> STDNAETGVIEAGNTDTDFSGELAAPGSNHTNVKFLFDRSRLLNVIKVLEKDAVFPRPFPTQEGAQQDDGYFCLLTPRPTVASRPATRFGLYANPSGSGVLANTSLDFNFYSLACFTYFRSDLEVTVVSLEPDLEFAVGWFPSGSEYQASSFVYDQLHVPFHFTGRTPRAFASKGGKVSFVLPWNSVSSVLPVRWGGASKLSSATRGLPAHADWGTIYAFVPRPNEKKSTAVKHVAVYIRYKNARAWCPSMLPFRSYK;> GPIPTAPRENSLMFLSTLPDDTVPAYGNVRTPPVNYLPGEITDLLQLARIPTLMAFERVPEPVPASDTYVPYVAVPTQFDDRPLISFPITLSDPVYQNTLVGAISSNFANYRGCIQITLTFCGPMMARGKFLLSYSPPNGTQPQTLSEAMQCTYSIWDIGLNSSWTFVVPYISPSDYRETRAITNSVYSADGWFSLHKLTKITLPPDCPQSPCILFFASAGEDYTLRLPVDCNPSYVF;> RVTTQTAGNTAINTQSSLGVLCAYVEDPTKSDPPSSSTDQPTTTFTAIDRWYTGRLNSWTKAVKTFSFQAVPLPGAFLSRQGGLNGGAFTATLHRHFLMKCGWQVQVQCNLTQFHQGALLVAMVPETTLDVKPDGKAKSLQELNEEQWVEMSDDYRTGKNMPFQSLGTYYRPPNWTWGPNFINPYQVTVFPHQILNARTSTSVDINVPYIGETPTQSSETQNSWTLLVMVLVPLDYKEGATTDPEITFSVRPTSPYFNGLRNRYTAG;> RGNNGNMTFNYYANTYQNSVDFSTSSSASGAGPGNSRGGLAGLLTNFSGILNPLGYLK

Seneca Valley virus (SVV) is an oncolytic picornavirus that selectively targets cancer cells by recognizing Tumor endothelial marker 8 (TEM8) as the host receptor. SVV has a typical picornavirus capsid with four capsid proteins; VP1, VP2, and VP3 are characterized by a single jelly roll fold, where eight beta-strands form a barrel-like structure that is distributed at the exterior of the virus, while VP4 is located on the interior of the capsid. The structural architecture consists of four capsid proteins forming a protomer, 5 protomers forming a pentamer, and 12 pentamers assembling into a pseudo T=3 capsid, approximately ~32 nm in diameter. We used cryo-electron microscopy to investigate SVV under acidic conditions and in complex with TEM8 at physiological pH, identifying multiple uncoating intermediates.

We also imaged SVV complexed with TEM8 under physiological conditions (pH 7 and 37°C). For both physiological and acidic conditions, the A-particles were resolved to 3.4 Å, while for the ER-particles, the resolutions were 6.4 and 4.3 Å, respectively. The A-particles obtained in both conditions are expanded by ~5% in diameter compared to the F-particle. This expansion results in reduced capsid protein contacts compared to the F-particle. Inter-pentamer contacts are reduced by 34% and 22% under acidic and physiological conditions, respectively. For the A-particle[P], additional disordered regions without interpretable density include VP1 (G13, S20, and S28), VP2 (D12), and VP3 (E61-S66), while for the A-particle[C], these include VP3 (P60-D67). On the capsid exterior, the A-particle[P] had the following partially ordered regions: the VP1 HI loop (S229), VP1 BC loop (A65), VP1 Loop II (G97), and VP2 residues V59 and D67, while the A-particle[C] exhibited similar behavior showing partially ordered regions: VP1 HI loop (T230) and VP1 Loop II (P95-G97). At the interior, the A-particle[P] displayed partially ordered regions in the VP1 N-terminus (S1-S28), VP2 N-terminus (R13-G20), VP3 FG loop (G160-N162), and VP4 N-terminus (S38, G63-K72). Interestingly, under physiological conditions, no receptor density is observed on the A-particle[P]. In the SVV A-particle, its genome is reorganized and lacks defined capsid-RNA interactions with the inner capsid surface, likely contributing to the flexibility of the VP1 N-terminus, which is consequently poorly resolved.>[2x]MGGFFARLKRSLLKTKENLGSGFISLFRGKKIDDDLFEELEEQLLIADVGVETTRKIITNLTEGASRKQLRDAEALYGLLKEEMGEILAKVDEPLNVEGKTPFVILMVGVNGVGKTTTIGKLARQFEQQGKSVMLAAGDTFRAAAVEQLQVWGQRNNIPVIAQHTGADSASVIFDAIQAAKARNIDVLIADTAGRLQNKSHLMEELKKIVRVMKKLDV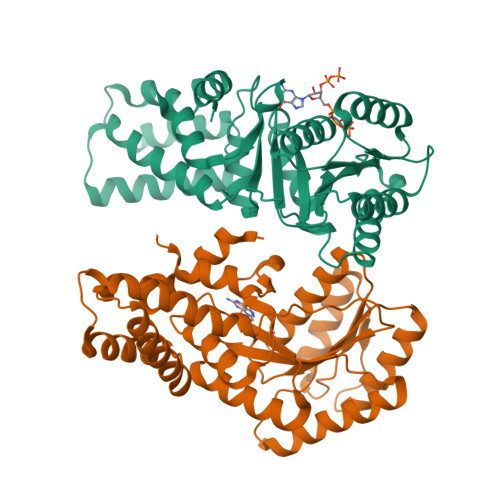EAPHEVMLTIDASTGQNAVSQAKLFHEAVGLTGITLTKLDGTAKGGVIFSVADQFGIPIRYIGVGERIEDLRPFKADDFIEALFAREDHHHHHH>MEKLHQCYWKSGEPQSDDIEASRMKRAAAKHLIERYYHQLTEGCGNEACTNEFCASCPTFLRMDNNAAAIKALELYKINAKLCDPHPSKKGASSAYLENSKGAPNNSCSEIKMNKKGARIDFKDVTYLTEEKVYEILELCREREDYSPLIRVIGRVFSSAEALVQSFRKVKQHTKEELKSLQAKDEDKDEDEKEKAACSAAAMEEDSEASSSRIGDSSQGDNNLQKLGPDDVSVDIDAIRRVYTRLLSNEKIETAFLNALVYLSPNVECDLTYHNVYSRDPNYLNLFIIVMENRNLHSPEYLEMALPLFCKAMSKLPLAAQGKLIRLWSKYNADQIRRMMETFQQLITYKVISNEFNSRNLVNDDDAIVAASKCLKMVYYANVVGGEVDTNHNEEDDEEPIPESSELTLQELLGEERRNKKGPRVDPLETELGVKTLDCRKPLIPFEEFINEPLNEVLEMDKDYTFFKVETENKFSFMTCPFILNAVTKNLGLYYDNRIRMYSERRITVLYSLVQGQQLNPYLRLKVRRDHIIDDALVRLEMIAMENPADLKKQLYVEFEGEQGVDEGGVSKEFFQLVVEEIFNPDIGMFTYDESTKLFWFNPSSFETEGQFTLIGIVLGLAIYNNCILDVHFPMVVYRKLMGKKGTFRDLGDSHPVLYQSLKDLLEYEGNVEDDMMITFQISQTDLFGNPMMYDLKENGDKIPITNENRKEFVNLYSDYILNKSVEKQFKAFRRGFHMVTNESPLKYLFRPEEIELLICGSRNLDFQALEETTEYDGGYTRDSVLIREFWEIVHSFAAEQKRLFLQFTTGTDRAPVGGLGKLKMIIAKNGPDTERLPTSHTAFNVLLLPEYSSKEKLKERLLKAITYAKGFGML[2x];>[2x]PQERPRKLPQLCTELQTTIHDIILECVYCKQQLLRREVYDFAFRDLCIVYRDGNPYAVCDKCLKFYSKISEYRHYSYSLYGTTLEQQYNKPLSDLLIRCINCQKPLSPEEKQRHLDKKQRFHNIRGRWTGRCMSC

Human protein E6AP/UBE3A, the founding member of the HECT-type ubiquitin ligase family, was originally identified as an associated partner of the viral oncoprotein E6 of human papillomaviruses (HPVs). The E6 oncoprotein from high-risk HPV types hijacks the ligase activity of the host E6AP to ubiquitinate the tumor suppressor p5313, leading to the aberrant p53 degradation. The HECT-type E3 ligases have a characteristic C-terminal HECT domain consisting of an N-lobe and a C-lobe that are responsible for E2 binding and ubiquitin acceptance, respectively. Here, by using cryogenic electronic microscopy, we reveal that the structures of full-length E6AP and E6AP/E6 complex are monomer and dimer of E6AP/E6 protomer, respectively.

After several rounds of 3D classification, we identified five distinct conformational states of the E6AP/E6 complex and resolved the structures of these five conformations at resolutions ranging from 2.6 to 4.4 Å. We therefore assigned the five conformations into one of two classes: attached (Att) or detached (Det). In all three Att conformations, the catalytic C-lobe of E6AP attaches to E6, whereas, in the two Det conformations, there are no interactions between the C-lobe and E6. We hereafter refer to the three Att conformations as Att1, Att2 and Att3 based on the distance between the tips of the two towers in a descending sequence: 74 Å in Att1, 71 Å in Att2, and 66 Å in Att3. Following the same nomenclature, the Det two conformations are referred to as Det1 (76 Å) and Det2 (61 Å). (2) When the two towers leant beyond a threshold, the Att conformation changed into a Det conformation. As the two towers underwent an outwards rotation, the Det2 conformation transformed into the Det1 conformation. Accompanying the E6AP/E6 complex conformational changes, there is substantial variation in the spatial relationship between the E6 from one protomer and the catalytic C-lobe of E6AP of the other protomer: far away (Det1), close (Det2), or in contact (Att). Since the interactions between the C-lobe and E6 do not exist in the Det conformations, these interactions are likely to be dispensable in terms of the dimerization of the E6AP/E6 protomer. The Det and Att conformations of the E6AP/E6 complex presented in this study should be structurally relevant to these accepting and donating processes, respectively. Unlike the N-lobe of E6AP, which is restricted by strong interactions with its N-terminal region, the C-lobe in the Det conformation is free to move around and accept ubiquitin from an E2; this is evident in the overlay structure of the HECT/E2–ubiquitin complex presented in Supplementary Fig. 14a.(2Z,6S)-6-{3-chloro-5-[5-(prop-1-yn-1-yl)pyridin-3-yl]thiophen-2-yl}-2-imino-3,6-dimethyltetrahydropyrimidin-4(1H)-one 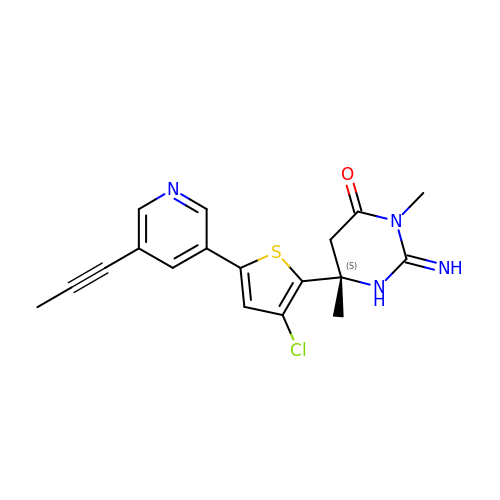| C18 H17 Cl N4 O S | IJYPXSRDUPWKPB-SFHVURJKSA-N One target protein for c‐di‐GMP is PilF, a hexameric ATPase from the thermophilic bacterium Thermus thermophilus important for pilus formation, cell motility, and DNA uptake from the environment. The N‐terminus of PilF contains three homologous so‐called general secretory pathway II (GSPII) domains, GSPII‐A, ‐B, and ‐C. Our recent structures of GSPII‐B (PilF159‐302) showed that the two nucleotide building blocks of c‐di‐GMP are recognized by the protein in a very similar manner through a duplicated amino acid sequence motif. In the GSPII‐B complex with c‐di‐GMP, both c‐di‐GMP phosphodiester groups accept a hydrogen bond from a backbone amide group of a conserved leucine (L168 from the first motif and L197 from the second motif) and from a side chain amino group of a conserved glutamine (Q190 from the first motif and Q218 from the second motif).

To gain insights into the structural basis for the pH‐dependent ligand recognition, we crystallized both the Q190E and the Q218E single‐site mutant of the PilF GSPII‐B domain in complex with c‐di‐GMP using very similar crystallization conditions at pH 7.0. Due to the high‐quality electron density maps for both mutants, their ligand recognition mode could be discerned in detail. In both the Q190E and the Q218E single point mutants, one phosphodiester‐binding pocket can be found in the mutant configuration and the other one in the WT configuration due to the duplication of the c‐di‐GMP phosphodiester binding motifs (Figure S2b‐e). Importantly, the carboxylate groups of the newly introduced glutamate sidechains in either of the two Q/E mutants were found to still point directly towards a non‐bridging oxygen atom of the phosphodiester groups for the carboxamide groups of the native glutamine side chains. The shortest distances between the oxygen atoms of the glutamate carboxylate groups and the phosphodiester groups were found to be 2.6 Å (Q190E) and 2.5 Å (Q218E), respectively, which is well below the sum of the van der Waals radii of the two oxygen atoms. Similarly, the hydrogen bond length between the L168 amide group and the phosphodiester oxygen in the Q218E mutant is increased by 0.2 Å compared to the native binding site in the Q190E construct (orange numbers). Finally, the lengths of the hydrogen bonds from E190 to the 2′‐OH group of c‐di‐GMP in the Q190E mutant and from E218 to the 2′‐OH group in the Q218E mutant are increased by 0.4 Å if compared to the native sites in both constructs (red numbers). While the c‐di‐GMP binding affinity of the WT protein is similar at pH 4.0 and 8.5 according to ITC titration experiments, both mutants display a drastic increase in ligand affinity at lower pH. Likewise, the KD of the Q218E mutant changed from ∼ 450 nM at pH 8.5 to ∼ 25 nM at pH 4.5. For the Q218E/c‐di‐GMP‐complex and the free Q218E protein, pKa values of 7.1 and 5.9 were determined.

>[2x]GSSGEGQKDLKLGELLLQKGWISREALEEALVEQEKTGDLLGRILVRKGLPEEALYRALAEEKGLEFLESTEGIVPDPSAALLLLRSDALRYGAVPIGFQNGEVEVVLSDPRHKEAVAQLLNRPARFYLALPQAWEELFRRAYPQK>ENEQYGANFNNADIRQFVEIVGQHLGKTILIDPSVQGTISVRSNDTFSQQEYYQFFLSILDLYGYSVITLDNGFLKVVRSANVKTSPGMIADSSRPGVGDELVTRIVPLENVPARDLAPLLRQMMDAGSVGNVVHYEPSNVLILTGRASTINKLIEVIKRVDVIGTEKQQIIHLEYASAEDLAEILNQLISESHGKSQMPALLSAKIVADKRTNSLIISGPEKARQRITSLLKSLDVEESEEGNTRVYYLKYAKATNLVEVLTGVSEKLKDEKGNARKPSSSGAMDNVAITADEQTNSLVITADQSVQEKLATVIARLDIRRAQVLVEAIIVEVQDGNGLNLGVQWANKNVGAQQFTNTGLPIFNAAQGVADYKKNGGITSANPAWDMFSAYNGMAAGFFNGDWGVLLTALASNNKNDILATPSIVTLDNKLASFNVGQDVPVLS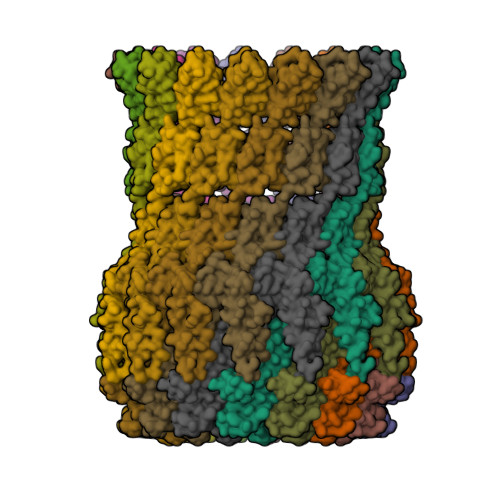GSQTTSGDNVFNTVERKTVGTKLKVTPQVNEGDAVLLEIEQEVSSVDSSSNSTLGPTFNTRTIQNAVLVKTGETVVLGGLLDDFSKEQVSKVPLLGDIPLVGQLFRYTSTERAKRNLMVFIRPTIIRDDDVYRSLSKEKYTRYRQEQQQRIDGKSKALVGSEDLPVLDENTFNSHAPAPSSR[15x]1,3-benzothiazole-6-sulfonamide | C7 H6 N2 O2 S2 | 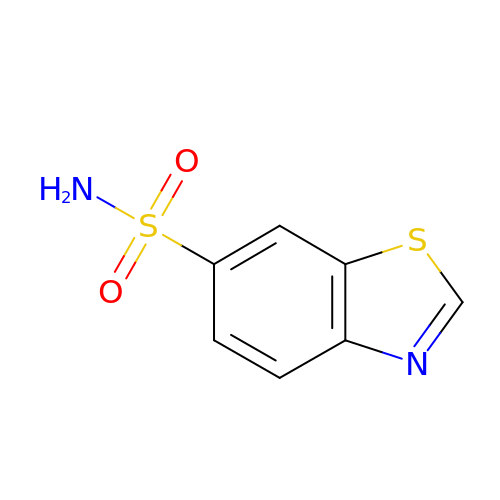KRRLILAOGRCMFH-UHFFFAOYSA-N> MAAESVRVAVRCRPFNQREKDLNTTLCVGMTPNVGQVNLNAPDGAAKDFTFDGAYFMDSTGEQIYNDIVFPLVENVIEGYNGTVFAYGQTGSGKTFSMQGIETIPAQRGVIPRAFDHIFTATATTENVKFLVHCSYLEIYNEEVRDLLGADNKQKLEIKEQPDRGVYVAGLSMHVCHDVPACKELMTRGFNNRHVGATLMNKDSSRSHSIFTVYVEGMTETGSIRMGKLNLVDLAGSERQSKTGATGDRLKEATKINLSLSALGNVISALVDGKSKHIPYRDSKLTRLLQDSLGGNTKTIMIACVSPSSDNYDETLSTLRYANRAKNIKNKPTINEDPKDALLREYQEEIARLKSMVQPGAVGPLEHHHHHH

OSM‐3 belongs to the homodimeric kinesin‐2 subfamily and is the Caenorhabditis elegans homologue of human KIF17. Similar to KIF17, OSM‐3 is involved in intraflagellar transport in the distal part of the cilium, and both proteins are autoinhibited at the resting state. The OSM‐3 motor domain shows the typical kinesin fold, with a central eight‐stranded β‐sheet surrounded by 3 α‐helices on either side. We have determined the structure of the motor domain of OSM‐3 either bound to ADP or to AMPPNP, or devoid of a nucleotide.

The best crystal diffracted X‐rays up to 2.1 Å resolution and was used in the analysis presented below. Although ATP was included in the purification buffer, ADP was found in the OSM‐3 nucleotide‐binding site, as is common with purified kinesins. Accordingly, the region from Arg238 to Lys254, which encompasses the C‐terminal part of the Switch 2‐containing L11 loop and the N‐terminal part of the neighboring α4 helix, is disordered. In addition, the L9 loop of ADP‐OSM‐3 is poorly ordered, with residues 195–201 unable to be built in the model, similar to, for example, the kinesin‐10 NOD but in contrast to the helical conformation found in other ADP‐kinesin structures. As this loop comprises the Switch 1 motif and is part of the nucleotide‐binding site, this observation agrees with a lower involvement of Switch 1 in the binding of ADP than of ATP. ADP and the associated Mg2+ ion are however tightly bound to OSM‐3, as reflected by their mean temperature factors (about 41 and 44 Å2, respectively) that are similar to that of the nearby P‐loop region (residues 86–96; 39 Å2), taken as a reference, but lower than that of the complete model (52 Å2). Another characteristic of ADP‐OSM‐3 is that the neck linker is docked onto the core motor domain, the ‘docked’ state being a feature of microtubule‐bound ATP‐kinesins. In the case of ADP‐OSM‐3, the movement of α4 might be facilitated because the two loops (L11 and L12) flanking α4 are mobile in this structure. In OSM‐3, this residue (Asn334) interacts with Asn80 and Asn295, similarly to what is observed in kinesin‐1. To sum up, the ADP‐OSM‐3 motor domain shows a standard structure of ADP‐kinesins.> GSMPVNNMVTG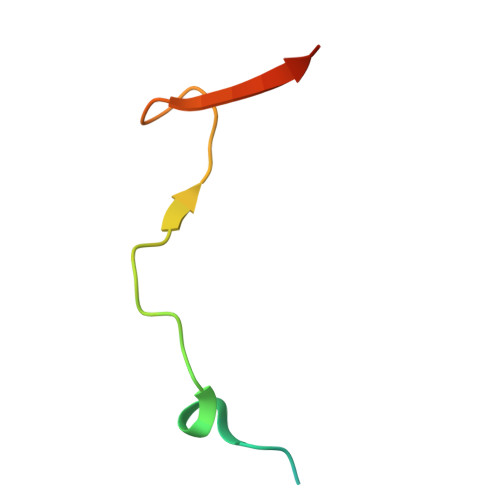YISIDAMKKFLGELHDFIPGTSGYLAYHVQNE Here, we carried out a structural and functional characterization of the TOSV cap-snatching endonuclease, an N terminal domain of the viral polymerase (L protein) that provides capped 3′OH primers for transcription. We report TOSV endonuclease crystal structures in the apo form, in complex with a di-ketoacid inhibitor (DPBA) and in an intermediate state of inhibitor release, showing details on substrate binding and active site dynamics. The structure has significant rearrangements in the domain folding compared to previously reported EN structures. To better illustrate these changes, we show the structure in comparison with the EN domain of the homologous LACV, the prototype of the Orthobunyavirus genus, in Figure 2B and C. The TOSV EN fold is organised as two alpha-beta lobes rather than the one alpha/beta and one alpha bundle lobe architecture that is conserved in LACV EN and all previously described bunyaviral cap-snatching EN structures. The active site of the TOSV EN is defined by the H-D-PD-E-K motif, and maintains the canonical configuration observed in other His+ cap-snatching ENs.

Crystals of the apo form grew as small bars in the presence of 2 mM MnCl2 that diffracted to 2.4 Å. In the apo crystal asymmetric unit, each molecule incorporates one Mn2+ ion (Mn1) in the active site with real space correlation coefficients (RSCC) of 1. The Mn2+ ions are octahedrally coordinated by the sidechains of D113 on βa, H78 on αb, E127 on βb and the main chain carboxyl of F128 on βb, together with two water molecules, all at distances of 2.2 Å. D90, residing in the flexible loop between αb and αc, is displaced from the manganese coordination site and shows high B-factors (above 94 Å2) compared to the low B-factors (<40 Å2) shown by the other highly ordered catalytic residues. The electron density for the entire flexible loop and in particular for D90 is weak but unambiguous for the main chain. K145 is located in helix αd, and forms one hydrogen bond to the water molecule that coordinates the manganese ion. The apo structure also contains seven sulphate ions bound to molA and three to molB in the asu with RSCC above 0.83. Four sulphate ions are found close to the active site. Since there are no cap-snatching EN structures in complex with RNA substrate available in the PDB, we explored the possibility that some of these sulphate ions could mimic the path of the TOSV EN RNA substrate binding. Finally, a fourth sulphate ion (SO4′), outside of the proposed RNA binding path, forms a hydrogen bond with K145 amino moiety. The amino acid sidechains involved in hydrogen bonds with these sulphate ions are conserved among Phenuiviridae ENs, with the sole exception of T131, further supporting that these sulphate ions are located in an RNA binding site (see alignment in Supplementary Figure S5).

>[2x]GMERILKKQPAPVRALTIHPLRRYESSIYDTPIPAYVIKHSSDGVTIDIATSELADGQSGSTIQPFESVPAQNLTLFKHDFTFGHLADTTDKKFVEVFGVLENRADDSDFQSPDMIIETETGHVYVVEFTTTMGDANSADLAARNKIAKYEIACLDRSAIKPISLYIIAVHFNGVVSNLDLSDEEVNEIVFRFRLARDIFEELREINPALFD>[4x]MKRMLINATQQEELRVALVDGQRLYDLDIESPGHEQKKANIYKGKITRIEPSLEAAFVDYGAERHGFLPLKEIAREYFPANYSAHGRPNIKDVLREGQEVIVQIDKEERGNKGAALTTFISLAGSYLVLMPNNPRAGGISRRIEGDDRTELKEALASLELPEGMGLIVRTAGVGKSAEALQWDLSFRLKHWEAIKKAAESRPAPFLIHQESNVIVRAFRDYLRQDIGEILIDNPKVLELARQHIAALGRPDFSSKIKLYTGEIPLFSHYQIESQ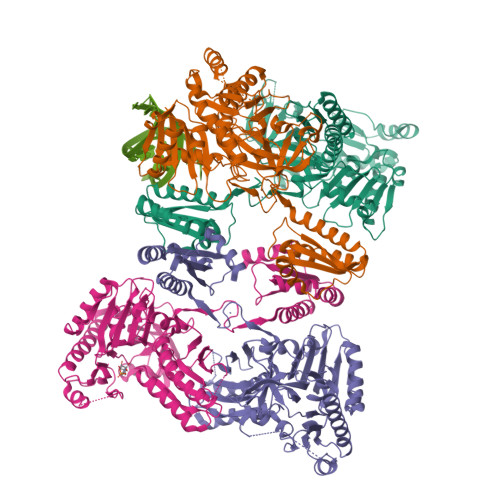IESAFQREVRLPSGGSIVIDSTEALTAIRINSARATRGGDIEETAFNTNLEAADEIARQLRLRDLGGLIVIRFIDMTPVRHQRAVENRLREAVRQDRARIQISHISRFGLLEMSRQRLSPSLGESSHHVCPRCSGTGTVRDNESLSLSILRLIEEEALKENTQEVHAIVPVPIASYLLNEKRSAVNAIETRQDGVRCVIVPNDQMETPHYHVLRVRKGEETPTLSYMLPKLHEEAM> VVEQSKICSSHYEPTV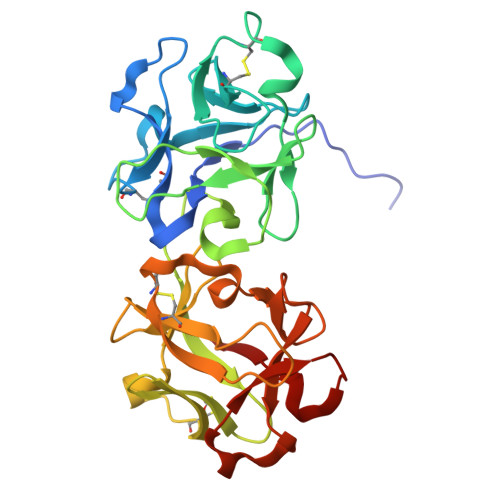RIGGRDGLCVDVSDNAYNNGNPIILWKCKDQLEVNQLWTLKSDKTIRSKGKCLTTYGYAPGNYVMIYDCSSAVAEATYWDIWDNGTIINPKSGLVLSAESSSMGGTLTVQKNDYRMRQGWRTGNDTSPFVTSIAGFFKLCMEAHGNSMWLDVCDITKEEQQWAVYPDGSIRPVQNTNNCLTCEEHKQGATIVMMGCSNAWASQRWVFKSDGTIYNLYDDMVMDVKSSDPSLKQIILWPYTGNANQMWATLF>PIVEIHLL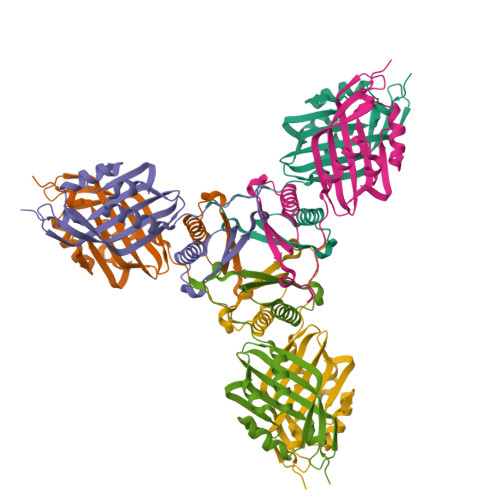EGYSDAEKERLGRSLTAAVQTVVPAPPEAITVMMHEMQAADYMRGATRRTPAPALPDAAATVRDFLDTMEARDLDKARTFLTDDFVMTFPTGRRMTDLSDLVEWSATRYRFVTKTYDRFDTAATLDGPVVYCFGTLRGEWPDGTPFDNVRFIDRFALRDGKLAVQDVWNDLEAMRPRG[6x]> MSRSKRDNNFYSVEIGDSTFTVLKRYQNLKPIGSGAQGIVCAAYDAILERNVAIKKLSRPFQNQTHAKRAYRELVLMKCVNHKNIIGLLNVFTPQKSLEEFQDVYIVMELMDANLSQVIQMELDHERMSYLLYQMLCGIKHLHSAGIIHRDLKPSNIVVKSDC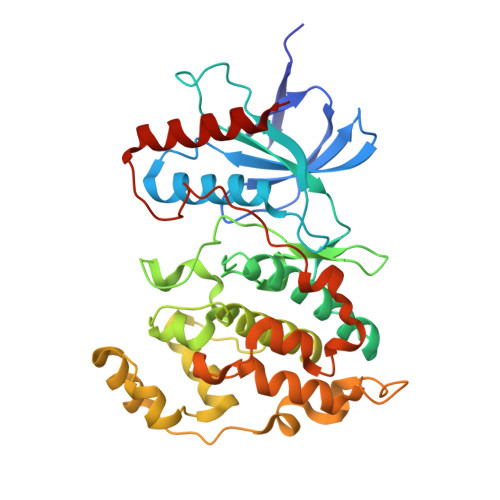TLKILDFGLARTAGTSFMMTPYVVTRYYRAPEVILGMGYKENVDIWSVGCIMGEMIKGGVLFPGTDHIDQWNKVIEQLGTPSPEFMKKLQPTVRTYVENRPKYAGYSFEKLFPDVLFPADSEHNKLKASQARDLLSKMLVIDASKRISVDEALQHPYINVWYDPSEAEAPPPKIPDKQLDEREHTIEEWKELIYKEVMDLEHHHHHH> NNWEQQKKNIEDDLDRYKKRAEELRKEAEKARKEARKTEDPTEEAKKEWEKRCKELEERARKLEDEAKDR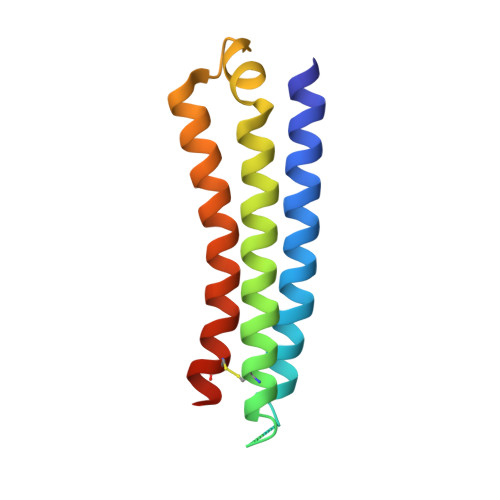VNDLFDSNFFQVIYSGDNDEEEWKKEKDRAEKEIEEWFKRIKEKCEEIKKRLEQ>MKIRDLLKARRGPLFSFEFFPPKDPEGEEALFRTLEELKAFRPAFVSITYGAMGSTRERSVAWAQRIQSLGLNPLAHLTVAGQSRKEVAEVLHRFVESGVENLLALRGDPPRGERVFRPHPEGFRYAAELVALIRERYGDRVSVGGAAYPEGHPESESLEADLRHFKAKVEAGLDFAITQLFFNNAHYFGFLERARRAGIGIPILPGIMPVTSYRQLRRFTEVCGASIPGPLLAKLERHQDDPKAVLEIGVEHAVRQVAELLEAGVEGVHFYTLNKSPATRMVLERLGLRPASGQPAKLAAALEHHHHHH[8x]

Methylenetetrahydrofolate reductase (MTHFR) is one of the key enzymes for production of methionine, which is not only an important amino acid precursor for protein synthesis, but also the precursor of S-adenosylmethionine (AdoMet), which serves as a major methyl donor and a substrate for polyamine synthesis. MTHFR uses NAD(P)H to reduce FAD; subsequently the reduced FAD reduces methylenetetrahydrofolate (CH2-H4folate). Here, we report biochemical properties and unique crystal structures of MTHFR from T. thermophilus HB8, one of the model organisms in structural biology. We demonstrate that the Thermus MTHFR is a dimer, rather than a tetramer, so that its symmetry is perhaps more directly relevant to the dimeric mammalian MTHFR.

The FAD-replete MTHFR in crystals was a homodimer of two holo-subunits. The FAD-replete MTHFR has one FAD cofactor per subunit, forming a dimer of holo-subunits. FAD treatment after purification not only contributed to the holo-subunit formation, but also dramatically altered the subunit contacts in the dimer. The large conformational change resulted from an ≈50° rotation of the apo-subunit relative to the holo-subunit upon FAD-binding. In the holo-dimer structure, a β-sheet was newly formed at the intermolecular interface, which was designated as β7'. A non-crystallographic two-fold axis is found between the β7' strands. In the FAD-replete MTHFR that was determined from crystals grown at pH 8.0, distances of Glu18(Oε)- His270(Nε), His270(Nδ)- Ser16(Oγ), and O4(ribityl chain of FAD)- Asp109 (Oε) were estimated as 2.98–3.06 Å, 2.95–3.30 Å and 2.58–2.71 Å, respectively. In our Thermus MTHFR structure, the Asp residue was 2.58–2.71 Å apart from the O4 of FAD in the ligand-free homodimer at pH 8.0, thus it was located in similar position of that of the NADH binding form of E. coli MTHFR. While the catalytic efficiency for the folate-dependent reaction of the homodimer is decreased to ∼50%, we observed that all flavin cofactors bound to the enzyme could be reduced by CH3-H4folate by the anaerobic titration. Since the lowered activities of Thermus MTHFR were exclusively found in the folate-dependent reactions, the positioning of Asp109 could be responsible.> MKPLVVFVLGGPGAGKGTQCARIVEKYGYTHLSAGELLRDERKNPDSQYGELIEKYIKEGKIVPVEITISLLKR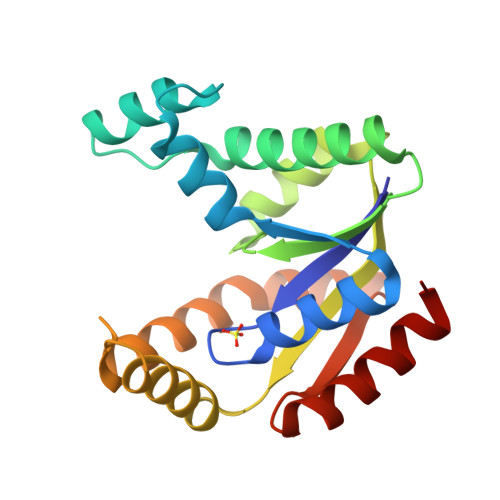EMDQTMAANAQKNKFLIDGFPRNQDNLQGWNKTMDGKADVSFVLFFDCNNEICIERCLERGKSSGRSDDNRESLEKRIQTYLQSTKPIIDLYEEMGKVKKIDASKSVDEVFDEVVQIFDKEG>[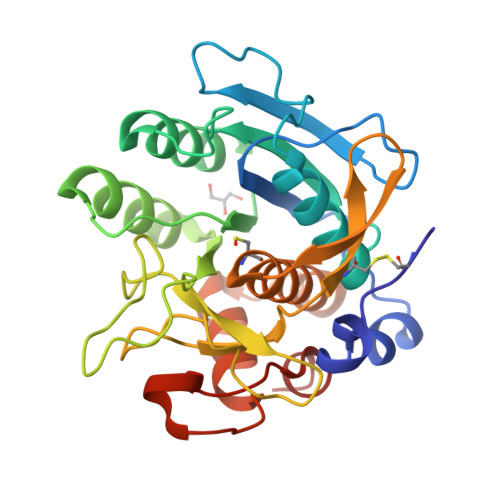3x]AKCVSYGVSQIKAPALHSQGYTGSNVKVAVIDSGIDSSHPDLNVAGGASFVPSETNPFQDNNSHGTHVAGTVLAVAPSASLYAVKVLGADGSGQYSWIINGIEWAIANNMDVINMSLGGPSGSAALKAAVDKAVASGVVVVAAAGNSGTSGSSSTVSYPAKYPSVIAVGAVDSSNQRAPWSSVGPELDVMAPGVSICSTLPGNKYGAHSGTCPASNHVAGAAALILSKHPNWTNTQVRSSLENTATKLGDSFYYGKGLINVEAAAQHHHHHH;> LPEGSPVTLDLRY> GKKSRVKTQKSGTGATATVSPKEILNLTSELLQKCSSPAPGPGKEWEEYVQIRTLVEKIRKKQKGLSVTFDGKREDYFPDLMKWASENGASVEGFEMVNFKEEGFGLRATRDIKAEELFLWVPRKLLMTVESAKNSVLGPLYSQDRILQA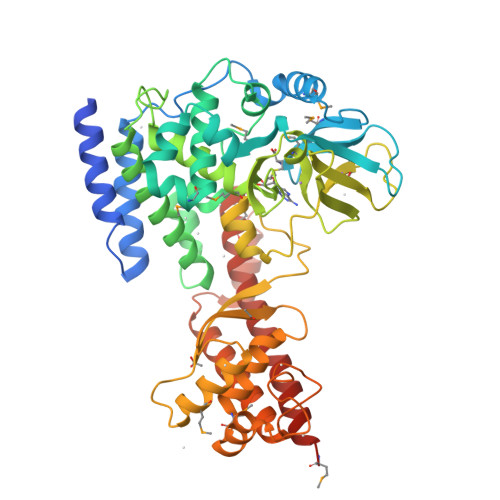MGNIALAFHLLCERASPNSFWQPYIQTLPSEYDTPLYFEEDEVRYLQSTQAIHDVFSQYKNTARQYAYFYKVIQTHPHANKLPLKDSFTYEDYRWAVSSVMTRQNQIPTEDGSRVTLALIPLWDMCNHTNGLITTGYNLEDDRCECVALQDFRAGEQIYIFYGTRSNAEFVIHSGFFFDNNSHDRVKIKLGVSKSDRLYAMKAEVLARAGIPTSSVFALHFTEPPISAQLLAFLRVFCMTEEELKEHLLGDSAIDRIFTLGNSEFPVSWDNEVKLWTFLEDRASLLLKTYKTTIEEDKSVLKNHDLSVRAKMAIKLRLGEKEILEKAVKSAAVNREYYRQQMEEKAP> AKKTPPVYPVTVPFLGHIVQFGKNPLEFMQRCKRDLKSGVFTISIGGQRVTIVGDPHEHSRFFSPRNEILSPREVYTIMTPVFGEGVAYAAPYPRMREQLNFLAEELTIAKFQNFVPAIQHEVRKFMAENWKEDE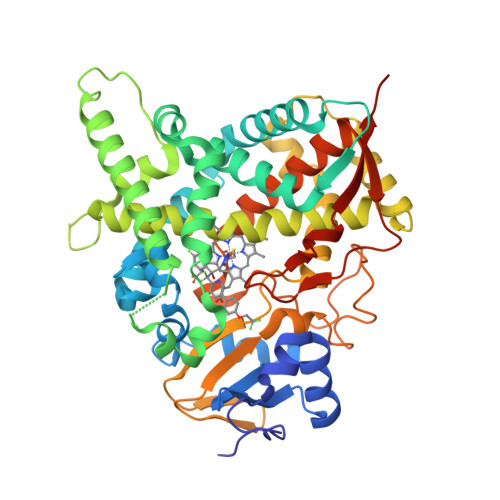GVINLLEDCGAMIINTACQCLFGEDLRKRLNARHFAQLLSKMESSLIPAAVFMPWLLRLPLPQSARCREARAELQKILGEIIVAREKEEASKDNNTSDLLGGLLKAVYRDGTRMSLHEVCGMIVAAMFAGQHTSTITTSWSMLHLMHPKNKKWLDKLHKEIDEFPAQLNYDNVMDEMPFAERCVRESIRRDPPLLMVMRMVKAEVKVGSYVVPKGDIIACSPLLSHHDEEAFPNPRLWDPERDEKVDGAFIGFGAGVHKCIGQKFALLQVKTILATAFREYDFQLLRDEVPDPDYHTMVVGPTLNQCLVKYTRKKKLPSHHHHHH> ITGTSTVGVGRGVLGDQKNINTTYSTYYYLQDNTRGDGIFTYDAKYRTTLPGSLWADADNQFFASYDAPAVDAHYYAGVTYDYYKNVHNRLSYDGNNAAIRSSVHYSQGYNNAFWNGSEMVYGDGDGQTFIPLSGGIDVVAHELTHAVTDYTAGLIYQNESGAINEAISDIFGTLVEFYANKNPDWEIGEDVYTPGISGDSLRSMSDPAKYGDPDHYSKRYTGTQDNGGVHINSGIINKAAYLISQGGTHYGVSVVGIGRDKLGKIFYRALTQYLTPTSNFSQLRAAAVQSATDLYGSTSQEVASVKQAFDAVGVK

We describe a device and a method for changing the ambient solution of a macromolecular crystal. Examples are given of the equilibration of three different crystals to new solutions with exchange times ranging from 5 to 180 min. In each case direct transfer of the crystal to the new solution causes cracking, which is eliminated with gradient equilibration using the described device. Crystals equilibrated with the device produce high-quality diffraction that yields refined structures comparable to those determined previously.

The structure was determined via molecular replacement to 1.75 Å resolution with a final refined Rwork and Rfree of 0.17 and 0.19, respectively. For the lysozyme and thermolysin crystals, just a 5 min gradient was sufficient to prevent visible cracking, while α-lactalbumin benefitted from more gradual treatments.2-[(3~{S},3'~{a}~{S},6'~{S},6'~{a}~{S})-6-chloranyl-6'-(3-chlorophenyl)-4'-(cyclopropylmethyl)-2-oxidanylidene-spiro[1~{H}-indole-3,5'-3,3~{a},6,6~{a}-tetrahydro-2~{H}-pyrrolo[3,2-b]pyrrole]-1'-yl]ethanoic 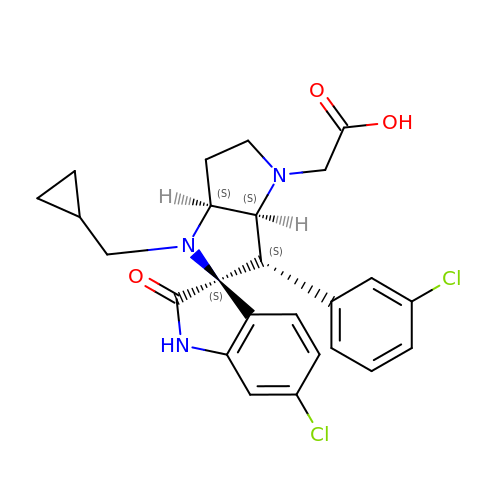acid | C25 H25 Cl2 N3 O3 | PECRYANCKVXSRI-FDHFVPJWSA-N>[4x]PEFFSVRHLELAGDDPYS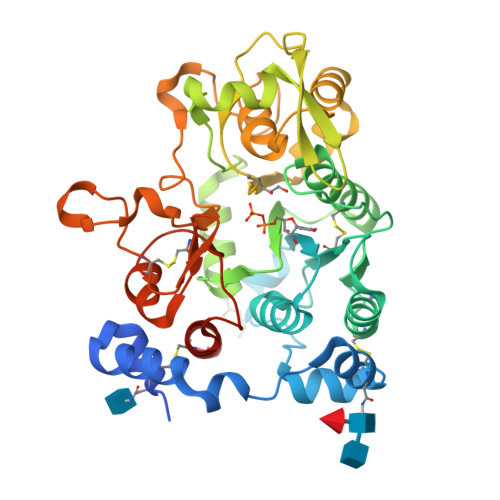NVNCTKILQGDPEEIQKVKLEILTVQFKKRPRWTPHDYINMTRDCASFIRTRKYIVEPLTKEEVGFPIAYSIVVHHKIEMLDRLLRAIYMPQNFYCIHVDRKAEESFLAAVQGIASCFDNVFVASQLESVVYASWTRVKADLNCMKDLYRMNANWKYLINLSGMDFPIKTNLEIVRKLKCSTGENNLETEKMPPNKEERWKKRYAVVDGKLTNTGIVKAPPPLKTPLFSGSAYFVVTREYVGYVLENENIQKLMEWAQDTYSPDEFLWATIQRIPEVPGSFPSSNKYDLSDMNAIARFVKWQYFEGDVSNGAPYPPCSGVHVRSVCVFGAGDLSWMLRQHHLFANKFDMDVDPFAIQCLDEHLRRKALENLEH The bacterial flagellar motor is a huge bidirectional rotary nanomachine that drives rotation of the flagellum for bacterial motility. The cytoplasmic C ring of the flagellar motor functions as the switch complex for the rotational direction switching from counterclockwise to clockwise. The basal body is made up of the LP ring, MS ring, C ring, rod and export apparatus. Here, we present two high-resolution cryo-electron microscopy structures of the C ring-containing flagellar basal body–hook complex from Salmonella Typhimurium, which are in the default counterclockwise state and in a constitutively active CheY mutant-induced clockwise state, respectively.

To obtain the C ring-containing basal body–hook complex in the CW state, we constructed the constitutively active double mutant D13K/Y106W of CheY (hereafter referred to as CheY**), which can mimic CheY-P to tightly bind to the C ring and lock the rotational direction of the motor in the CW state. The C ring-containing basal body–hook complex in the CW state was obtained by incubating the recombinant CheY** protein with the above purified basal body–hook complex in the CCW state. Further local refinement on four protomers with the symmetry-expanded particles improved the density map to a resolution of 4.4 Å. CheY** is bound into an open groove between two adjacent protomers on the surface of the middle subring of the C ring and interacts with FliGM, FliMM and the prior FliMM domain. At the interface with FliM, CheY** interacts with FliMM and the N-terminal loop and the αN helix of FliMN. The α1 helix, L2, L6, L8 and L10 loops of CheY** form an open concave surface to interact with loopα2–β3, loopα3–α4, loopβ5–α5 and α5 of FliMM. The mutated residue D13K of CheY** interacts with the loopα3–α4 of FliMM, while the mutated residue Y106W is located on the α4–β5–α5 surface of CheY** and stacks with the αN helix of FliMN, suggesting that the double mutation activates CheY through generating direct interactions with the C ring. In the interactions with FliG, the L6 and L8 loops of CheY** clamp the α11 helix of FliGM. CheY** also contacts with the β2, β6 and β7 strands and the linking loopβ6–β7 of FliMM–1 of the prior protomer via its α1–β2 surface, which enhances the inter-protomer interactions in the middle subring. The binding of CheY** also induces a significant contraction of the loop LMC that connects FliGM and FliGCN and results in the formation of an elongated HelixMC, which not only reduces the distance between FliGM and FliGCN by ~7 Å, but also causes a CW rotation of FliGCN by ~28° on the binding surface of the FliGM–1 domain in the prior protomer.

>MSDMNNPSDENTGALDDLWADALNEQKATTTKSAADAVFQQLGGGDVSGAMQDIDLIMDIPVKLTVELGRTRMTIKELLRLTQGSVVALDGLAGEPLDILINGYLIAQGEVVVVADKYGVRITDIITPSERMRRLSR[9x];>[3x]MSATASTATQPKPLEWLNRLRANPRIPLIVAGSAAVAIVVAMVLWAKTPDYRTLFSNLSDQDGGAIVAQLTQMNIPYRFANGSGAIEVPADKVHELRLRLAQQGLPKGGAVGFELLDQEKFGISQFSEQVNYQRALEGELARTIETLGPVKSARVHLAMPKPSLFVREQKSPSASVTVTLEPGRALDEGQISAVVHLVSSAVAGLPPGNVTLVDQSGHLLTQSNTSGRDLNDAQLKFANDVESRIQRRIEAILSPIVGNGNVHAQVTAQLDFANKEQTEEHYSPNGDASKATLRSRQLNISEQVGAGYPGGVPGALSNQPAPPNEAPIATPPTNQQNAQNTPQTSTSTNSNSAGPRSTQRNETSNYEVDRTIRHTKMNVGDIERLSVAVVVNYKTLADGKPLPLTADQMKQIEDLTREAMGFSDKRGDTLNVVNSPFSAVDNTGGELPFWQQQSFIDQLLAAGRWLLVLVVAWILWRKAVRPQLTRRVEEAKAAQEQAQVRQETEEAVEVRLSKDEQLQQRRANQRLGAEVMSQRIREMSDNDPRVVALVIRQWMSNDHE;>MGDSILSQAEIDALLNGDSDTKDEPTPGIASDSDIRPYDPNTQRRVVRERLQALEIINERFARQFRMGLFNLLRRSPDITVGAIRIQPYHEFARNLPVPTNLNLIHLKPLRGTGLVVFSPSLVFIAVDNLFGGDGRFPTKVEGREFTHTEQRVINRMLKLALEGYSDAWKAINPLEVEYVRSEMQVKFTNITTSPNDIVVNTPFHVEIGNLTGEFNICLPFSMIEPLRELLVNPPLENSRHEDQNWRDNLVRQVQHSELELVANFADIPLRLSQILKLKPGDVLPIEKPDRIIAHVDGVPVLTSQYGTVNGQYALRVEHLINPILNSLNEEQPK[3x];>MSNLSGTDKSVILLMTIGEDRAAEVFKHLSTREVQALSTAMANVRQISNKQLTDVLSEFEQEAEQFAALNINANEYLRSVLVKALGEERASSLLEDILETRDTTSGIETLNFMEPQSAADLIRDEHPQIIATILVHLKRSQAADILALFDERLRHDVMLRIATFGGVQPAALAELTEVLNGLLDGQNLKRSKMGGVRTAAEIINLMKTQQEEAVITAVREFDGELAQKIIDEMFLFENLVDVDDRSIQRLLQEVDSESLLIALKGAEPPLREKFLRNMSQRAADILRDDLANRGPVRLSQVENEQKAILLIVRRLAETGEMVIGSGEDTYV[3x];>MADKELKFLVVDKFSTMRRIVRNLLKELGFNNVEEAEDGVDALNKLQAGGFGFIISDWNMPNMDGLELLKTIRADSAMSALPVLMVTAEAKKENIIAAAQAGASGWVVKPFTAATLEEKLNKIFEKLGM[3x]>[2x]MTSPSHASDRGGGDGDSVENQSPELRKDPVTNRWVIFSPARAKRPTDFKSKSPQNPNPKPSSCPFCIGREQECAPELFRVPDHDPNWKLRVIENLYPALSRNLETQSTQPETGTSRTIVGFGFHDVVIESPVHSIQLSDIDPVGIGDILIA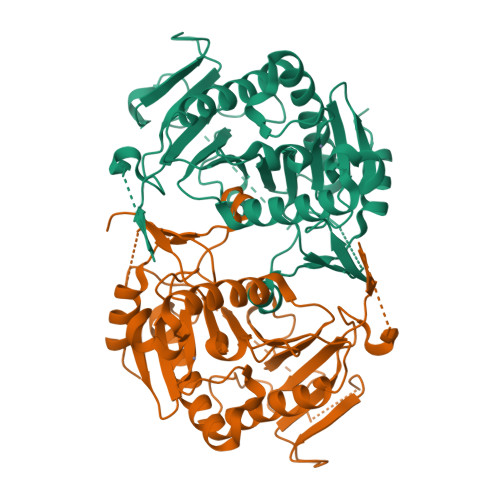YKKRINQIAQHDSINYIQVFKNQGASAGASMSHSHSQMMALPVVPPTVSSRLDGTKDYFEETGKCCLCEAKSKHFVIDESSHFVSVAPFAATYPFEIWIIPKDHSSHFHHLDDVKAVDLGGLLKLMLQKIAKQLNDPPYNYMIHTSPLKVTESQLPYTHWFLQIVPQLSGVGGFEIGTGCYINPVFPEDVAKVMREVSLT>GGMGQTLLDALNVRVVGSGERVLVLAHGFGTDQSAWNRILPFFLRDYRVVLYDLVCAGSVNPDFFDFRRYTTLDPYVDDLLHILDALGIDQCAYVGHSVSAMIGILASIRRPELFSKLILIGASPRFLNDEDYHGGFEQGEIEKV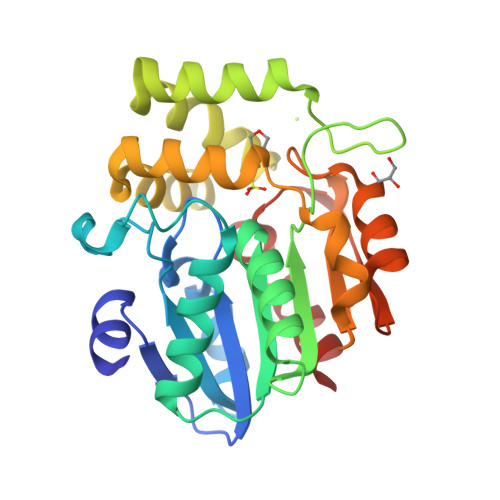FSAMEANYEAWVNGFAPLAVGADVPAAVREFSRTLFNMRPDITLFVSRTVFNSDMRGVLGLVKVPCHIFQTARDHSVPASVATYLKNHLGGKNTVHWLIIEGHLPHLSAPTLLAQELRRALSHR[2x]> MASSSSLVPDRLRLPLCFLGVFVCYFYYGILQEKITRGKYGEGAKQETFTFALTLVFIQCVINAVFAKILIQFFDTARVDHTRSWLYAACSISYLGAMVSSNSALQFVNYPTQVLGKSCKPIPVMLLGVTLLKKKYPLAKYLCVLLIVAGVALFMYKPKKVVGIEEHTVGYGELLLLLSLTLDGLTGVSQDHMRAHYQTGSNHMMLNINLWSTLLLGMGILFTGELWEFLSFAERYPAIIYNILLFGLTSALGQSFIFMTVVYFGPLTCSIITTTRKFFTILASVILFANPISPMQWVGTVLVFLGLGLDAKFGKGAKKTSHGENLYFQ

The endoplasmic reticulum (ER) cannot synthesize ATP but must import cytoplasmic ATP to energize protein folding, quality control and trafficking. Here we report that human SLC35B1 does not bind nucleotide sugars but indeed executes strict ATP/ADP exchange with uptake kinetics consistent with the import of ATP into crude ER microsomes. We have further determined seven cryogenic electron microscopy structures of human SLC35B1 in complex with an Fv fragment and either bound to an ATP analogue or ADP in all major conformations of the transport cycle. We conclude that SLC35B1 operates by a stepwise ATP translocation mechanism, which is a previously undescribed model for substrate translocation by an SLC transporter.

The SLC35B1–Fv–MBP fusion complex was optimized for cryo-EM with or without the addition of the non-hydrolysable ATP analogue adenylyl imidodiphosphate (AMP–PNP), which was first confirmed to produce equivalent STD NMR signals and transport activity as ATP. SLC35B1 structures with and without AMP–PNP addition are mostly equivalent, apart from the extra cryo-EM map density for the nucleotide. Unexpectedly, the ring-shaped map density implied a nucleotide conformation where the terminal γ-phosphate had arched back towards the adenine moiety. However, this is an unusual configuration for the ATP analogue, and the symmetrical map density made it difficult to confidently assign its correct orientation. The Q113F mutant structure adopted the same conformation as the wild-type structure but with minor side-chain differences located around the phenylalanine residue introduced in the cavity-closing contacts. The map density for AMP–PNP in Q113F was in the same position as in wild-type SLC35B1; however, the improved resolution now enabled its unambiguous assignment and confirmed the toroid shape conformation of the ATP analogue.>[2x]MGSSHHHHHHHSSGLVPRGSHMTEPVKLSGPMLPAVSGAAKSLVVLLHGYGSDGRDLIALGQFWRDSFPDTMFVAPNAPHVCGGNPF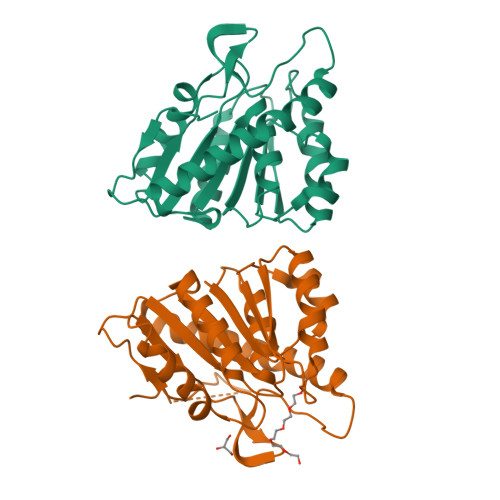GYEWFPLDLERDRTLARLAGAETAHPVLDAFLADLWAQTGLGPADTILVGFSQGAMMALYTGLRLPEPLKAIIAFSGLIVAPEKLEAEIASKPPVLLIHGDLDDVVPVIGSETALPKLIDLGIDARLHISQGSGHTIAQDGLDTATAFLREIL> GSHMTRLAPVVVDVPDDVLVLRVIGPLFFAAAEGLFTDLESRLEGKRIVILKWDAVPVLDAGGLDAFQRFVKRLPEGCELRVCNVEFQPLRTMARAGIQPIPGRLAFFPNRRAAMADL;> MSTIEERVKKIIGEQLGVKQEEVTNNASFVEDLGADSLDT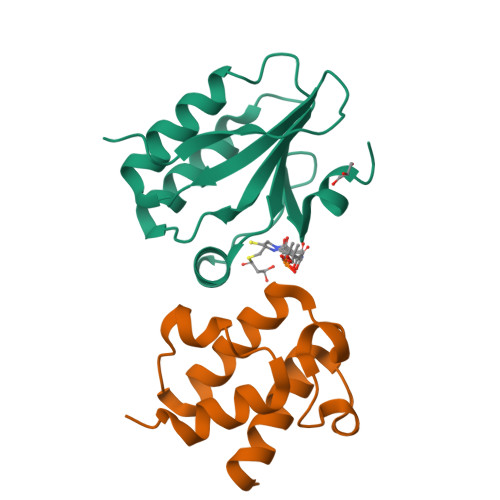VELVMALEEEFDTEIPDEEAEKITTVQAAIDYINGHQA> RSWHYVEPKFLNKAFEVALKVQIIAGFDRGLVKWLRVHGRTLSTVQKKALYFVNRRYMQTHWANYMLWINKKIDALGRT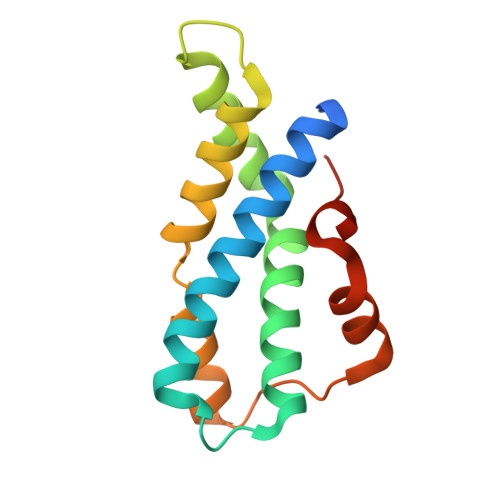PVVGDYTRLGAEIGRRIDMAYFYDFLKDKNMIPKYLPYMEEINRMRPADVPVKYMGK> M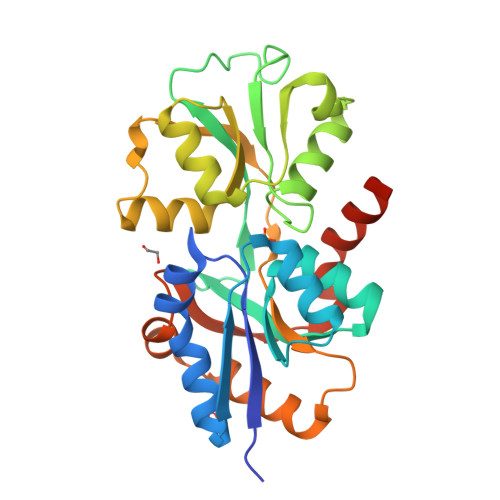AEVVNGKLHLRFAIAPMRPTPSQTIKEFEPIFKYLADQLGATYEIVSPESWAAISVAMTNGHVDVGWLGPWGYVLSNKKAGTEVLATVKYRGEPFYKALIVGRADLPIKKWPEDAKGLKLSLSDQGNTSGWLIPMAYFKSIGIDPASYFEYREGATFGQNESQIQHGLIDLGSDMDRGRNGMIEAGQIDPSKSKIVWESSKLPNDAISVPKDFDPALKARITEILTSLSEEKAQSLMGSGYNGFVKAKHSDYKVIEDAGRILGKLLEHHHHHH(8alpha)-17-(pyridin-3-yl)androsta-4,16-dien-3-one | C24 H29 N O | 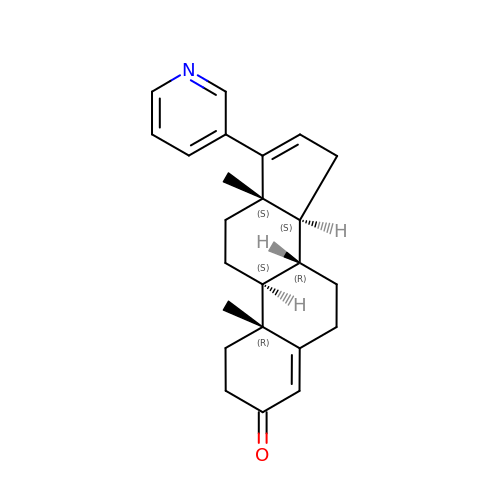GYJZZAJJENTSTP-NHFPKVKZSA-N> SSD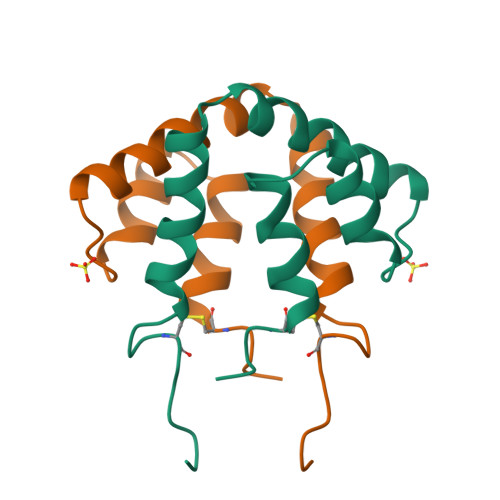ICPGFLQVLEALLLGSESNYEAALKPFNPASDLQNAGTQLKRLVDTLPQETRINIVKLTEKILTSPLCEQDLRV>MSLRIDVDTNFP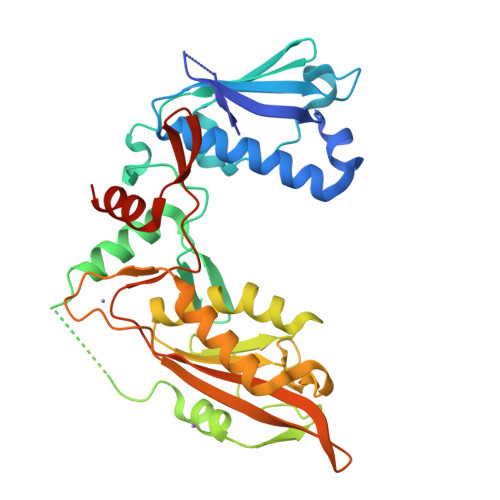ECVVDAGKVTLGTQQRQEMDPRLREKQNEIILRAVCALLNSGGGIIKAEIENKGYNYERHGVGLDVPPIFRSHLDKMQKENHFLIFVKSWNTEAGVPLATLCSNLYHRERTSTDVMDSQEALAFLKCRTQTPTNINVSNSLGPQAAQGSVQYEGNINVSAAALFDRKRLQYLEKLNLPESTHVEFVMFSTDVSHCVKDRLPKCVSAFANTEGGYVFFGVHDETCQVIGCEKEKIDLTSLRASIDGCIKKLPVHHFCTQRPEIKYVLNFLEVHDKGALRGYVCAIKVEKFCCAVFAKVPSSWQVKDNRVRQLPTREWTAWMMEADHHHHHH[2x]>GSPEFMALTQSLKLSNGVMMPV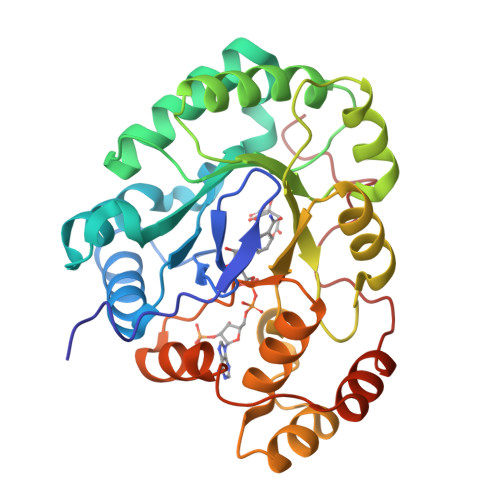LGFGMWKLQDGNEAETATMWAIKSGYRHIDTAAIYKNEESAGRAIASCGVPREELFVTTKLWNSDQGYESTLSAFEKSIKKLGLEYVDLYLIHWPGKDKFIDTWKAFEKLYADKKVRAIGVSNFHEHHIEELLKHCKVAPMVNQIELHPLLNQKALCEYCKSKNIAVTAWSPLGQGHLVEDARLKAIGGKYGKTAAQVMLRWEIQAGVITIPKSGNEARIKENGNIFDFELTAEDIQVIDGMNAGHRYGPDPEVFMNDF[2x]>[4x]MKSLQALFG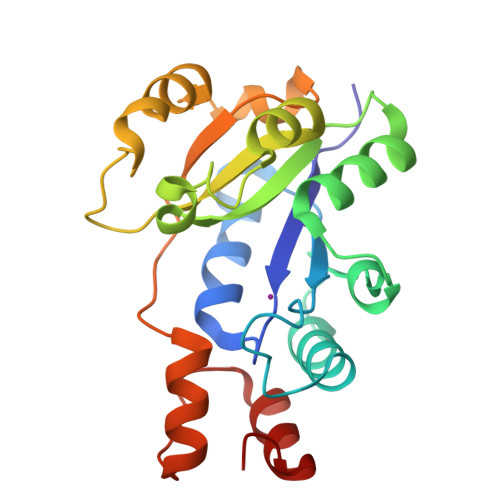GTFDPVHYGHLKPVETLANLIGLTRVTIIPNNVPPHRPQPEANSVQRKHMLELAIADKPLFTLDERELKRNAPSYTAQTLKEWRQEQGPDVPLAFIIGQDSLLTFPTWYEYETILDNAHLIVCRRPGYPLEMAQPQYQQWLEDHLTHNPEDLHLQPAGKIYLAETPWFNISATIIRERLQNGESCEDLLPEPVLTYINQQGLYR~{N}-[(1~{S})-2-[(4-methoxy-2,5-dimethyl-phenyl)methylamino]-1-[4-(3-oxidanylprop-1-ynyl)phenyl]ethyl]-5-methyl-1,2-oxazole-3-carboxamide | C26 H29 N3 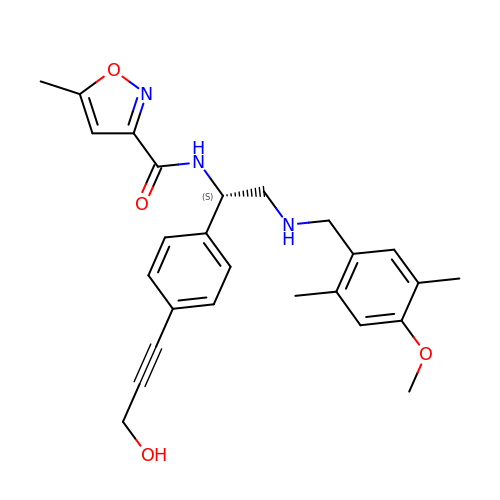O4 | DNHSLHQHJBUNLI-XMMPIXPASA-N N-dodecylmethanethioamide 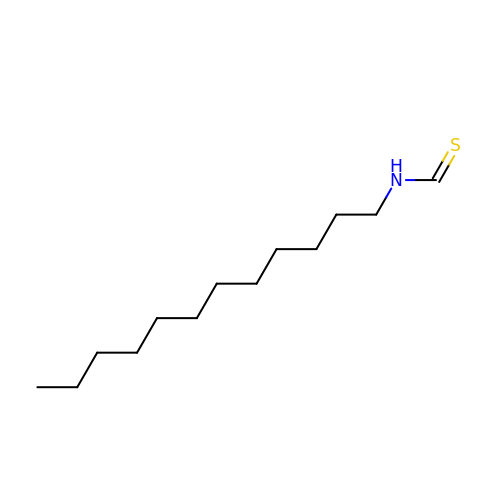| C13 H27 N S | BDXCOJKIHNDCOM-UHFFFAOYSA-N(R)-4-((4-((6-(2-(2,4-difluorophenyl)-1,1-difluoro-2-hydroxy-3-(1H-tetrazol-1-yl)propyl)pyridin-3-yl)ethynyl)phenoxy)methyl)benzonitrile 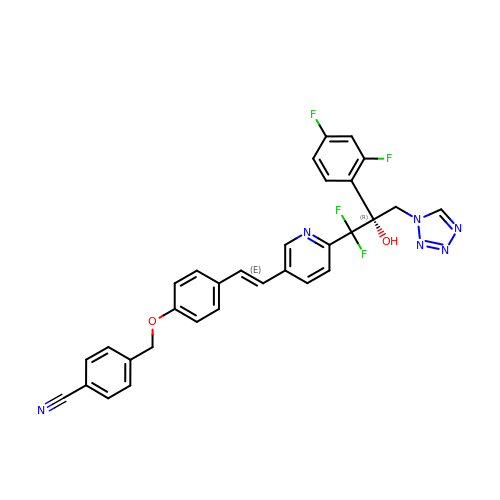| C31 H22 F4 N6 O2 | CHNOUXLXTKTWQU-PMERELPUSA-N> SHMTNLQTFELPTEVTGCAADISLGRALIQAWQKDGIFQIKTDSEQDRKTQEAMAASKQFCKEPLTFKSSCVSDLTYSGYVASGEEVTAGKPDFPEIFTVCKDLSVGDQRVKAGWPCHGPVPWPNNTYQKSMKTFMEELGLAGERLLKLTALGFELPINTFTDLTRDGWHHMRVLRFPPQTSTLSRGIGAHTDYGLLVIAAQDDVGGLYIRPPVEGEKRNRNW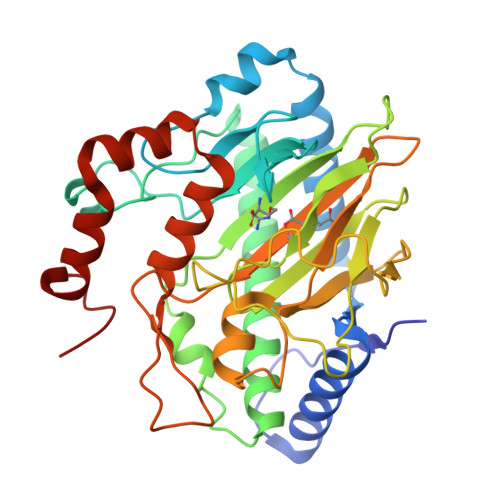LPGESSAGMFEHDEPWTFVTPTPGVWTVFPGDILQFMTGGQLLSTPHKVKLNTRERFACAYFHEPNFEASAYPLFEPSANERIHYGEHFTNMFMRCYPDRITTQRINKENRLAHLEDLKKYSDTRATGS> GSHMKISARNVFKGTVSALKEGAVNAEVDILLGGGDKLAAVVTLESARSLQLAAGKEVVAVVKAPWVLLMTDSSGYRLSARNILTGTVKTIETGAVNAEVTL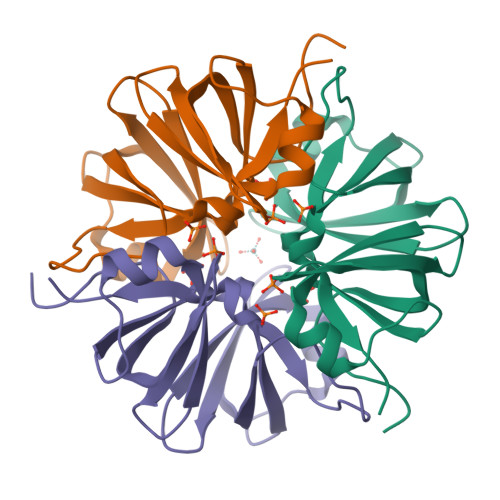ALQGGTEITSMVTKEAVAELGLKPGASASAVIKASNVILGVPA> ARLGRQALLFPLCLVLYEFSTYIGNDMIQPGMLAVVEQYQAGIDWVPTSMTAYLAGGMFLQWLLGPLSDRIGRRPVMLAGVVWFIVTCLAILLAQNIEQFTLLRFLQGISLCFIGAVGYAAIRESFEEAVCIKITALMANVALIAPLLGPLVGAAWIHVLPWEGMFVLFAALAAISFFGLQRAMPETATRIGEKLSLKELG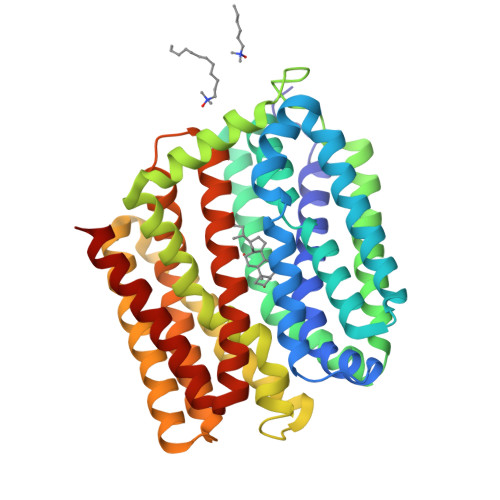RDYKLVLKNGRFVAGALALGFVSLPLLAWIAQSPIIIITGEQLSSYEYGLLQVPIFGALIAGNLLLARLTSRRTVRSLIIMGGWPIMIGLLVAAAATVISSHAYLWMTAGLSIYAFGIGLANAGLVRLTLFASDMSKGTVSAAMGMLQMLIFTVGIEISKHAWLNGGNGLFNLFNLVNGILWLSLMVIFLK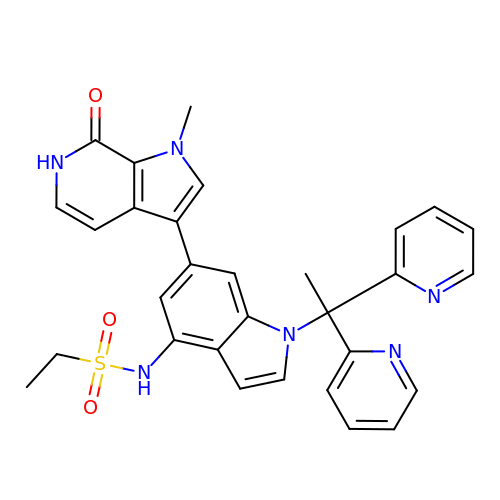N-{1-[1,1-di(pyridin-2-yl)ethyl]-6-(1-methyl-7-oxo-6,7-dihydro-1H-pyrrolo[2,3-c]pyridin-3-yl)-1H-indol-4-yl}ethanesulfonamide | C30 H28 N6 O3 S | LMLIBNUOIWAJFC-UHFFFAOYSA-N> EDGGS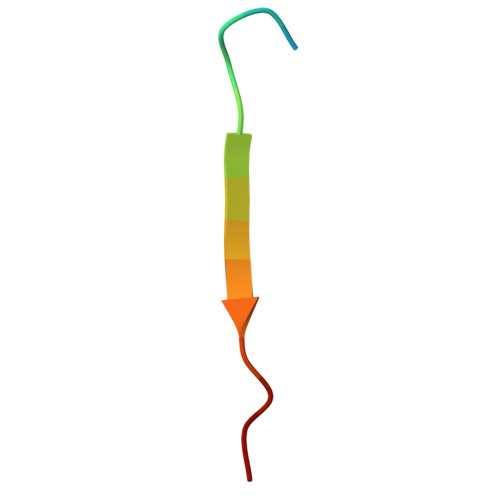SWEYIWTLPSG>[2x]MGEELNRLLDVLGNETRRRILFLLTKRPYFVSELSRELGVGQKAVLEHLRILEEAGLIESRVEKIPRGRPRKYYMIKKGLRLEILLT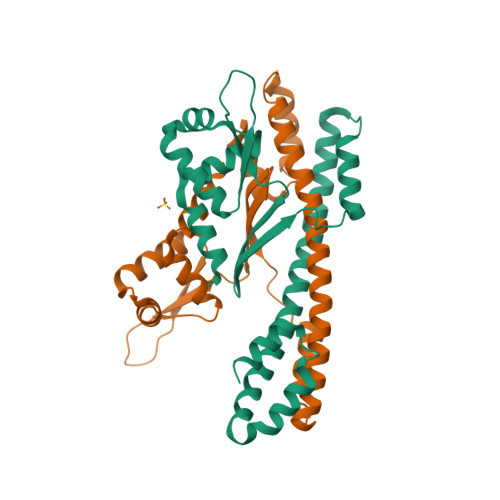PTLFGSEMYEAKGVRKSPEYEQAKELIKSQEPINVKMRELAEFLHELNERIREIIEEKRELEEARILIETYIENTMRRLAEENRQIIEEIFRDIEKILPPGYARSLKEKFLNINI ID30A-3 (or MASSIF-3) is a mini-focus (beam size 18 µm × 14 µm) highly intense (2.0 × 1013 photons s−1), fixed-energy (12.81 keV) beamline for macromolecular crystallography (MX) experiments at the European Synchrotron Radiation Facility (ESRF). MASSIF-3 is recommended for collecting diffraction data from single small crystals (≤15 µm in one dimension) or for experiments using serial methods.

In a first experiment, we collected diffraction data from a Se-Met derivatized crystal of ferulic acid esterase (FAE; Prates et al., 2001) with the aim of de novo structure determination using the SAD technique (f′′ = 3.7 e− at 12.834 keV). The transmitted white beam then impinges on a liquid-nitro­gen-cooled single Si(111) crystal with a bandwidth of 1.5 × 10−4 used as a monochromator for MASSIF-3, which delivers a beam at a photon energy of 12.812 keV into its experimental hutch (EH2). This energy on the high-energy remote side of the selenium edge was chosen in order to be able to use the anomalous scattering contribution from selenium for de novo phasing experiments. Data were measured according to a strategy proposed by an EDNA characterization at 100 K from a crystal cryo-protected using Paratone N and were automatically processed. Subsequent de novo phasing performed with hkl2map and SHELXC/D/E found all 16 Se sites (8 per chain), and automatic building with ARP/WARP resulted in a model containing 280 and 281 residues (out of 297 residues) for the two FAE monomers in the asymmetric unit which was then further refined using Coot and refmac5.

>MASDKFPVAENPSSSFKYESAVQYRPAPDSYLNPCPQAGRIVKETYTGINGTKSLNVYLPYGYDPNKKYNIFYLMHGGGENENTIFSNDVKLQNILDHAIMNGELEPLIVVTPTFNGGNCTAQNFYQEFRQNVIPFVESKYSTYAESTTPQGIAASRMHRGFGGFSMGGLTTWYVMVNCLDYVAYFMPLSGDYWYGNSPQDKANSIAEAINRSGLSKREYFVFAATGSEDIAYANMNPQIEAMKALPHFDYTSDFSKGNFYFLVAPGATHWWGYVRHYIYDALPYFFHELEHHHHHH[2x]>SSGMQ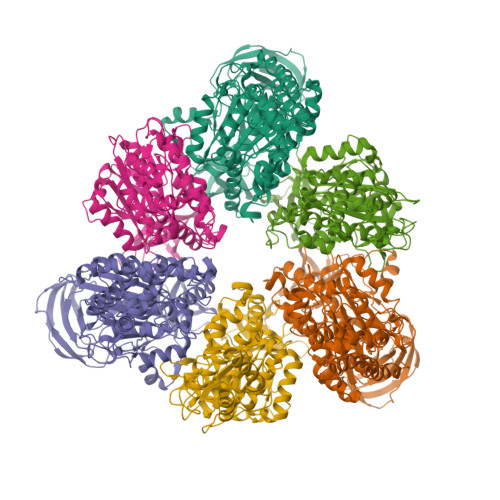IGKIIKVSGPLVMAENMSEASIQDMCLVGDLGVIGEIIEMRQDVASIQVYEETSGIGPGEPVRSTGEALSVELGPGIISQMFDGIQRPLDTFMEVTQSNFLGRGVQLPALDHEKQWWFEATIEEGTEVSAGDIIGYVDETKIIQHKIMVPNGIKGTVQKIESGSFTIDDPICVIETEQGLKELTMMQKWPVRRGRPIKQKLNPDVPMITGQRVIDTFFPVTKGGAAAVPGPFGAGKTVVQHQIAKWSDVDLVVYVGCGERGNEMTDVVNEFPELIDPNTGESLMERTVLIANTSNMPVAAREASIYTGITIAEYFRDMGYDVAIMADSTSRWAEALREMSGRLEEMPGDEGYPAYLGSRLAEYYERSGRVIALGSDQREGSITAISAVSPSGGDISEPVTQNTLRVVKVFWGLDSSLAQKRHFPSINWIQSYSLYSTEVGRYMDQILQQDWSDMVTEGMRILQEEEQLNEIVRLVGIDSLSDNDRLTLEVAKSIREDYLQQNAFDDVDTFTSREKQFNMLKVILTFGKEARKALSLGAYFNEIMEGTVAVRERISRSKYIPEEELAKISSINEEIKETIQLIVSEGGMTDD[3x];>[3x]MIKEYRTIKEVVGPLMAVEKVSGVKYEELIEVRMQNGEIRRGQVLEVQEDKAMVQIFEGTSGINLKNSSVRFLGHPLQLGVSEDMIGRVFDGLGRPKDNGPEILPEKYLDINGEVINPIARDYPDEFIQTGISAIDHLNTLVRGQKLPVFGPPGAGKSALAAQIARQATVLDSSDDFAVVFAAIGITFEEAEFFMEDFRQTGAIDRSVMFMNLANDPAIERIATPRMALTAAEYLAYEKGMHVLVIMEDMTNYAEALREISAARREVPGRRGYPGYLYTNLATLFERAGRIRGLKGSVTQIPILTMPEDDKTHPIPDLTGYITEGQIILTRELYKSGISPPIDVLPSLSRLKDKGTGAGKTREDHAATMNQLFAAYAQGKQAKELAVVLGESALSDIDKIYAKFAERFENEYVNQGFYTNRTITETLDLGWELLAMLPRTELKRIKDDLLDKYLPEGK>HMLNVGATAPDFTLRDQNQQLVTLRGYRGAKNVLLVFFPLAFTGICQGELDQLRDHLPEFENDDSAALAISVGPPPTHKIWATQSGFTFPLLSDFWPHGAVSQAYGVFNEQAGIANRGTFVVDRSGIIRFAEMKQP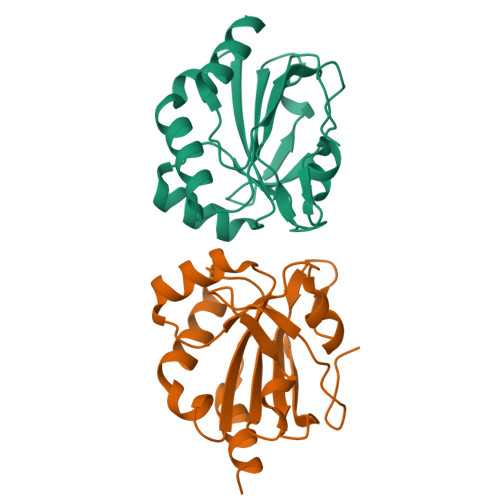GEVRDQRLWTDALAALTA[4x]>GPEGSKTFNIPTFVLDENCNFIPDVLSRANAKFIKEVLIRDSYNAVCLANSFIPMATQTVEQILIIITKFKFSRSRDLLMSVFRLGVHINRFYAGKNQVKHMITMMKSLFDTEEAMRQLDRALMGLFVDARDNSYMPLIALSLHENGLPDSKFIKAVRLIQTTVNSFHNRPDADIEQYAEKLRAYNYLYKIPKYTLKEAVDIYSDNLKDLTIGVNKKPTLLFTSSDDAYLSHIYNDLLFLTSTWNMIYNCKKEIRRLNTWIKYEINSIMETAVLVGFQLPDLKETILDLAALISNMNLVSPDKELFPHYKLILAKLFEICIF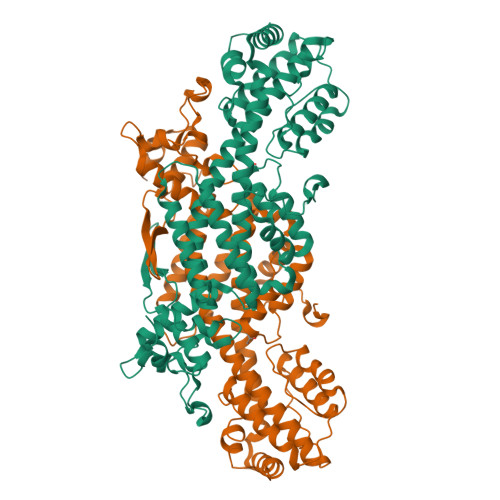ATKANICILPSFIKGHLIEFEDVLKRSNDDEDLNYLLLKSRDSDDEYDEDKPPIQVDPGRVDNVLTDSDFFNVTPENAFSSIAIMPISYDKTIDVEDNEIQVLEVEMQSLSAVVYGAVASKYGLSLEQVIRKLNQNE[2x]>GHMNDALHIGLPPFLVQANNEPRVLAAPEARMGYVLELVRANIAADGGPFAAAVFERDSGLLIAAGTQRVVPGRCSAAHAEILALSLAQAKLDTHDLSADGLPACELVTSAEPCVMCFGAVIWSGVRSLVCAARSDD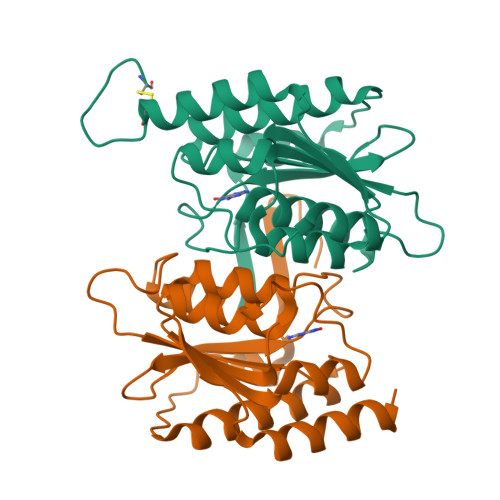VEAIGFDEGPRPENWMGGLEARGITVTTGLLRDAACALLREYNACNGVIYNARCGVHK[2x]>ASMTGGQQMGAPITAYAQQTRGLLGCIITSLTGRDKNQVEGEVQIVSTATQTFLATCINGVCWTVYHGAGTRTIASPKGPVIQMYTNVDQDLVGWPAPQGSRSLTPCTCGSSDLYLVTRHADVIPVRRRGDSRGSLLSPRPISYLKGSSGGPLLCPTGHAVGLFRAAVCTRGVAKAVDFIPVENLETTMRGSHHHHHH[2x];>KKGSVVIVGR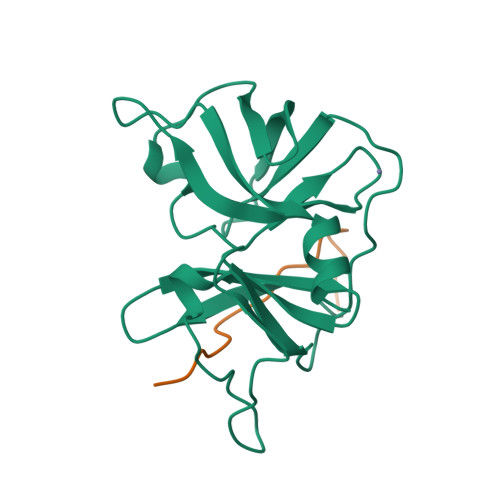IVLSGKPAIIPKK[2x]> CVHAEEASSTGRNFNVEKINGEWHTI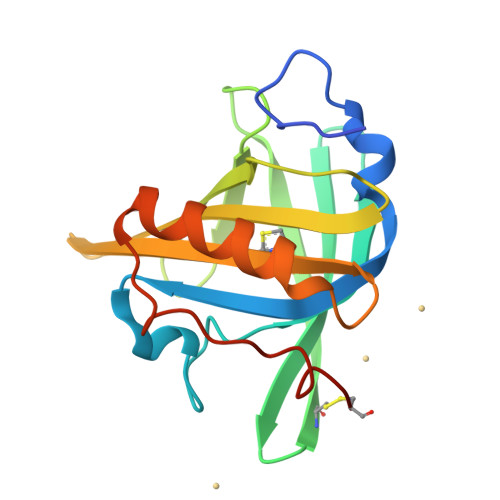ILASDKREKIEDNGNFRLFLEQIHVLENSLVLKFHTVRDEECSELSMVADKTEKAGEYSVTYDGFNTFTIPKTDYDNFLMAHLINEKDGETFQLMGLYGREPDLSSDIKERFAQLCEEHGILRENIIDLSNANRCLQARE>[2x]MARYLVVAHRTAKSPELAAKLKELLAQDPEARFVLLVPAVPPPGWVYEENEVRRRAE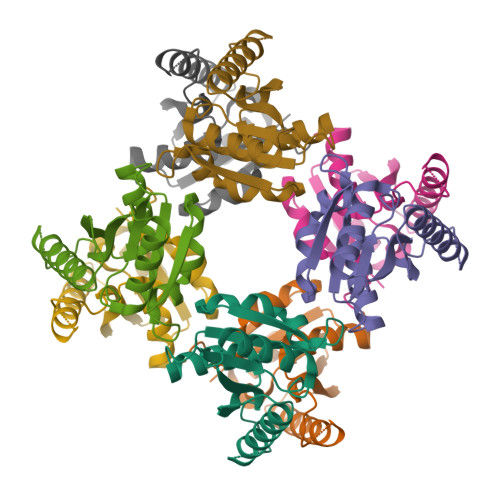EEAAAAKRALEAQGIPVEEAKAGDISPLLAIEEELLAHPGAYQGIVLSTLPPGLSRWLRLDVHTQAERFGLPVIHVIAQAA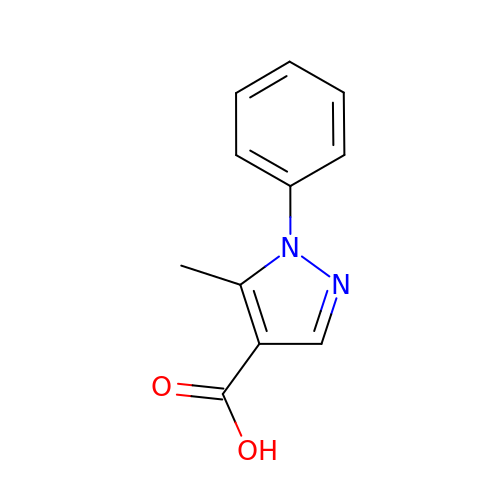5-methyl-1-phenyl-pyrazole-4-carboxylic acid | C11 H10 N2 O2 | USSMIQWDLWJQDQ-UHFFFAOYSA-N> MTPEAIIEDRRFQETLDKIRKEEGYDFAAIAFYESNKPSSPIKWHYVSGN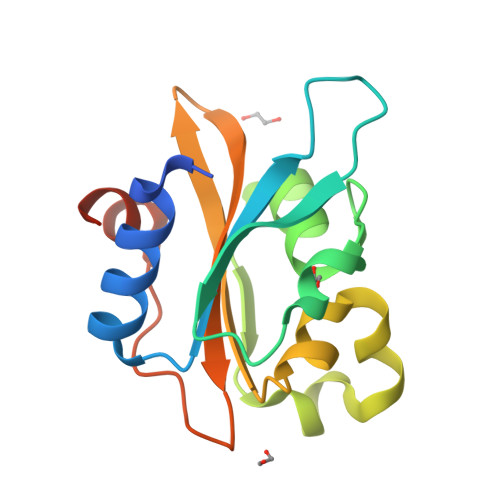KNNRFKLIILRKGRGLAGTVMKTGKRMVIANVGLALGPEEKIDAPILLSESLTAVLAVPLWYKNQVYGVLLFGQRDGRPLPKIFDNDDIQRKFGIFNDDK>GSQIHVDTMKVINDPIHGHIELHPLLVRIIDTPQFQRLRYIKQLGGGYYVFPGASHNRFEHSLGVGYLAGCLVHALGEKQPELQISERDVLCV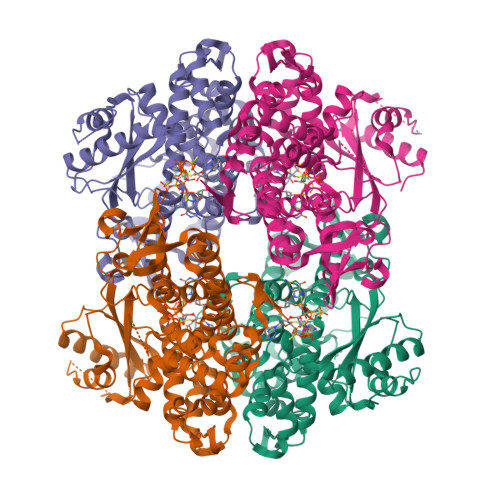QIAGLCHDLGHGPFSAMFDGRFIPLARPEVKWTHEQGSVMMFEHLINSNGIKPVMEQYGLIPEEDICFIKEQIVGPLESPVEDSLWPYKGRPENKSFLYEIVSNKRNGIDVDKWDYFARDCHHLGIQNNFDYKRFIKFARVCEVDNELRICARDKEVGNLYDMFHTRNSLHRRAYQHKVGNIIDTMITDAFLKADDYIEITGAGGKKYRISTAIDDMEAYTKLTDNIFLEILYSTDPKLKDAREILKQIEYRNLFKYVGETQPTGQIKIKREDYESLPKEVASAKPKVLLDVKLKAEDFIVDVINMDYGMQEKNPIDHVSFYCKTAPNRAIRITKNQVSQLLPEKFAEQLIRVYCKKVDRKSLYAARQYFVQWCADRNFTKPQDGDVIAPLITPQKKEWNDSTSVQNPTRLREASKSRVQLFKDDPM[8x]> GPMARTFILWLHGLGDSGPANEPIQTQFKSSELSNASWLFPSAPFNPVTCNNGAVMRSWFDVPELPFKVGSPIDESSVLEAVKNVHAIIDQEIAEGTNPENVFICGLSQGGALTLASVLLYPKTLGGGAVLSGWVPFTSSIISQFPEEAKKTPILWSHGTDDRMVLFEAGQAALPFLKEAGVTCEFKAYPGLGHSISNKELKYIESWIKRRLKGSSSTCLQLNCLKEMFH

To elucidate the molecular features encoded by these conserved elements, we solved the crystal structures of Arabidopsis thaliana SOBER1 and Zea mays B6T1C9, each representing a different clade in the phylogenetic tree. Both proteins fold into a canonical α/β hydrolase architecture and superpose with a root-mean-square deviation (RMSD) of atomic positions of 1.54 Å over 210 amino acid residues. We found that a loop constituting the hydrophobic tunnel lid is the major component determining substrate turnover rate and substrate specificity.

Similar to the crystal structure of ZmB6T1C9/ZmAPT2, we discovered a substrate tunnel in the AtSOBER1 protein, though severely impaired by a two amino acid insertion (LP63-64) into the loop that constitutes the tunnel lid. We found one insertion (L63) to directly block the entrance to the tunnel. The insertion of the second-amino acid (P64) pushes the following residue (F65) into the tunnel, which is positioned in the middle of the hydrophobic tunnel and could act as a hydrophobic anchor for the lid. The two amino acid insertion is conserved within the entire family clade, well aligning with the leucine at the tunnel entrance and the phenylalanine in the center of the tunnel, the latter of which is in most cases a phenylalanine or a leucine. In contrast to Zea mays acyl-protein thioesterase 2 and in agreement with Cunnac et al. (2007), Arabidopsis SOBER1 displayed a clear preference for pNP acetate. We found B-factors of the loop as low as the rest of the protein in AtSOBER1, and increased B-factors in the acyl-protein thioesterases APT1 and ZmB6T1C9/ZmAPT2. This indicated that in AtSOBER1 all protein parts retained a similar rigidity, whereas in APT1 and ZmB6T1C9/ZmAPT2 the loop had a higher flexibility than the rest of the protein. As previously reported, AtSOBER1 repressed AvrBsT-elicited HR, while its paralog (which we named AtTIPSY1) did not. Subsequent incubation of acetylated AvrBsT with purified AtSOBER1 led to hydrolysis of 14C-acetyl-AvrBsT. Altogether, our experiments reveal that AtSOBER1 is a protein deacetylase.>GGSVKQLEDKVEELLSKNAHLENEVARLKKLQKQMSKKMNDQLELMESNIRRDIRQGFVDLQTEKSDLIDNVGAIPFLDYKHFASRIFFPEAGTLTAVMIRDIGEDSEQTTVDEKCLAFAELIRDKQFLSCFVHALEEQKNFSIKDKCTVASLLTLALHGDLLYLTEIMEDLLQSLMDQSSNANPKLLLRRTESIVEKLLTNWMSICLYGFLRESVGQPLFLLVSALTQQISKGPVDSVTEKALYTLSEDWLLCQAQDFEPLKLKVVFAVGTGEEISESLEVIALTCDTIQQVKEKILQTFQRKFGFRYTQQIRDIEIEYEKEGKFV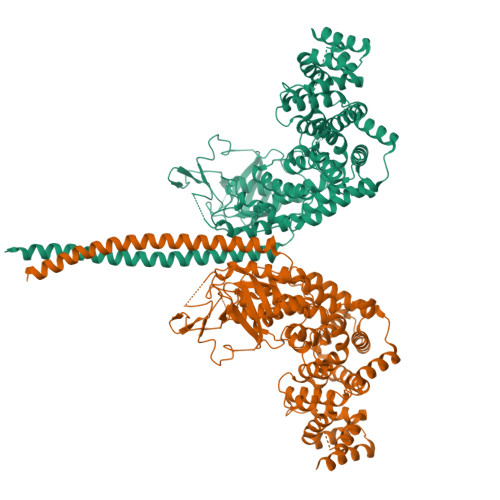MLQEVDDTSEIRGHVTMLNTLKHYQVGDGACIKVITPKIHAPLKTQNSVKDDKNFSIKYFHLVDPDIDTDLSNHPEKKALKIKEMYLIKLLSTKVAVHSFVENLFKSIWGLPNNKAPLAVKYFFDFLDEQAERKKITDPDVLHIWKTNSLPLRFWVNILKNPDFVFSDMEKSPHLDGCLSVIAQAFMDSFSLTDTHLDKHSPTNKLLYGKDIPQYKQEVKSYYKLVKDQTSISSQELKTFLQEESKKHQNEFNESAALRELYKYMQRYFTEIFQKLEQTDAPSNLKENMHRVKELFDNMKRSGWN[2x]> ECQPIFLNVLEAIEPGVVCAGHDNNQPDSFAALLSSLNELGERQLVHVVKWAKALPGFRNLHVDDQMAVIQYSWMGLMVFAMGWRSFTNVNSRMLYFAPDLVFNEYRMHKSRMYSQCVRMRHLSQEFGWLQIT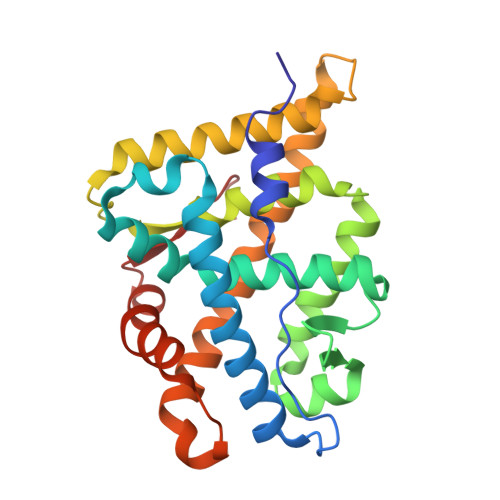PQEFLCMKALLLFSIIPVDGLKNQKFFDELRMNYIKELDRIIACKRKNPTSCSRRFYQLTKLLDSVQPIARELHQFTFDLLIKSHMVSVDFPEMMAEIISVQVPKILSGKVKPIYFHTQ>MEALKIALLGGGTVGSAFYNLVLERAEELSAFGVVPRFLGVLVRDPR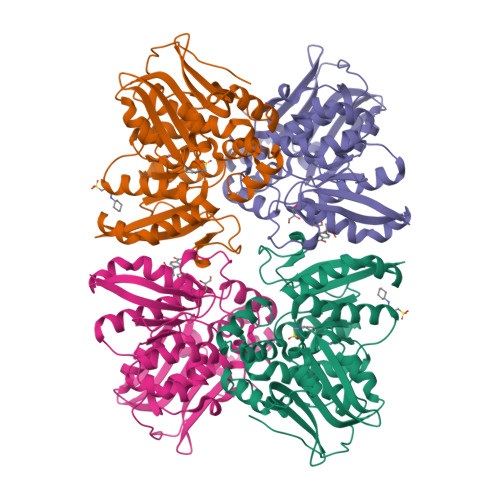KPRAIPQELLRAEPFDLLEADLVVEAMGGVEAPLRLVLPALEAGIPLITANKALLAEAWESLRPFAEEGLIYHEASVMAGTPALSFLETLRGSELLELHGILNGTTLYILQEMEKGRTYAEALLEAQRLGYAEADPTLDVEGIDAAHKLTLLARLLVDPGFPFAEVEAQGIARLTPEVLQKAEARGERVRLVASLFGEGGRWRAAVAPRRLPQDHPLARARGNALWVRARPLGEAFVTGPGAGGGATASGLFADLLRFLSGAPGHLPAPRARPPLEEGSPWPGVE[2x]>MLPRPSGTYAGLPIADYGDAPPLSTKTMFWRTSPEKLPPGAWEPAYLGSKDERVDGPSLQQVMRDQLKPYSEPRGLLPPQEILDAVCDAIENRLENTLEPQKPWTFKKACESLDKNTSSGYPYHKQKSKDWTGSAFIGDLGDQATHANNMYEMGKSMRPIYTAALKDELVKPDKIYGKIKKRLLWGSDLGTMIRAARAFGPFCDALKETCIFNPIRVGMSMNEDGPFIFARHANFRYHMDADYTRWDSTQQRAILKRAGDIMVRLSPEPDLARVVMDDLLAPSLLDVGDYKIVVEEGLPSGCPCTTQLNSLAHWILTLCAMVEVTRVDPDIVMQESEFSFYGDDEVVSTNLELDMVKYTMALRRYGLLPTRADKEEGPLERRQTLQGISFLRRAIVGDQFGWYGRLDRASIDRQLLWTKGPNHQNPFETLPGHAQRPSQLMALLGEAAMHGEKYYRTV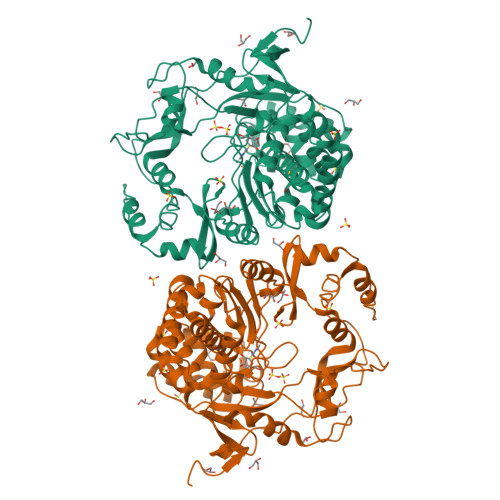ASRVSKEAAQSGIEMVVPRHRSVLRWVRFGTMDAETPQERSAVFVNEDAAALEHHHHHH[3x]>[2x]MGSSHHHHHHSSGLMITPIISSNLGLKHRVTLRKATLASLMQSLSGESSNRVMWNDRYDTLLIARDPREIKNAIEKSVTDFGGLENYKELTGGADPFALMTPVCGLSANNIFKLMTEKDVPIDPTSIEYLENTSFAEHVNTLDSHKNYVVIVNDGRLGHKFLIDLPALTQGPRTAYIIQSDLGGGALPAVRVEDWISRRGSDPVSLDELNQLLSKDFSKMPDDVQTRLLASILQIDKDPHKVDIKKLHLDGKLRFASHEYDFRQFQRNAQYVAGLG

One family of T3S effectors, the Cifs, re-program the host cell cycle causing arrest at the G2/M or the G1/S transition. In this study the crystal structures of Cif from P. luminescences (CifPl) and B. pseudomallei (CifBp) are presented. The structures reveal a head-and-tail domain arrangement, with the head-domain adopting an overall fold similar to papain-like cysteine proteases. The structure of the tail-domain of CifPl and CifBp presents an extensive surface area adjacent to the active site suggestive of a binding surface for interaction with a specific substrate.

Limited protelysis of CifBp with trypsin identified a stable fragment with a molecular weight of ∼30 kDa, as determined from SDS-PAGE gels (not shown). MALDI-TOF analysis of this CifBp fragment is most consistent with digestion of the protein following Arg55 (PINNACLE Lab., Newcastle University). Therefore, CifBp may in fact start at Met61 and amino acid numbering in this study reflects this (i.e. the sequence numbering begins at M(1)ITPIISSNLG). Although it is expected that Cif proteins function as monomers in vivo, each of the Cifs produced in this study displays the properties of monomer-dimer equilibria in solution, with the exception of CifBp which purifies as a single species (whose apparent molecular weight suggests a dimeric form). The two chains of CifBp overlay with an rmsd of 0.42 Å (245 equivalent Cα atoms) and can therefore be considered essentially identical. The structure of CifBp determined here is virtually identical to that recently determined independently. The tail-domain of CifBp (back to residue 14) adopts a conformation very similar to that found in CifPl, even though there is very little sequence identity between these proteins in this region. The structure of CifPl overlays on CifBp with rmsds of 1.24 Å (chain A, 226 equivalent Cα atoms) and 1.25 Å (chain B, 226 equivalent Cα atoms). CifPl and CifBp overlay on the structure of CifEc (chain A) with an rmsd of 1.33 Å and 1.20 Å respectively (145 and 151 equivalent Cα atoms). The structures presented here show that the conformation of the occluding loop is conserved in both CifPl (residues 203–212) and CifBp (residues 168–177).>HEHNTIPKGASIEVKVQQLDPVNGNKDVGTVTITESNYGLVFTPDLQGLSEGLHGFHIHENPSCEPKEEEGKLTAGLGAGGHWDPKGAKQHGYPWQDDAHLGDLPALTVLHDGTATNPVLAPRLKHLDDVRGHSIMIHTGGDNHSDHPAPLG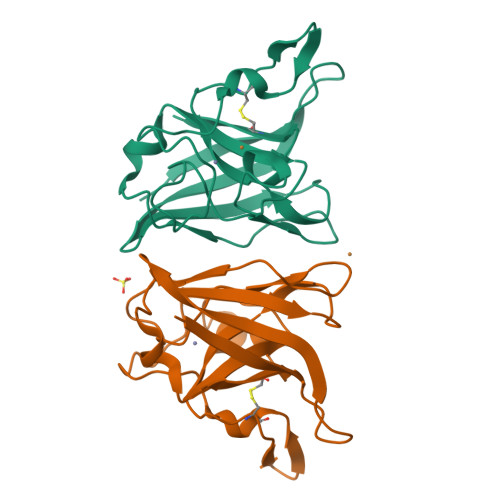GGGPRMACGVIK[3x]> HHHHVKLSVVEQAPVVEGLTPAHSLQHSIELARLADRLGYERFWVAEHHAEIFNAVPAPEILIARIAAETSGIRVGSGGVLLSLYSPLKVAEVFRTLHALYPDRIDLGIGRANRVKLPVFAALRDDTAGKEPSSD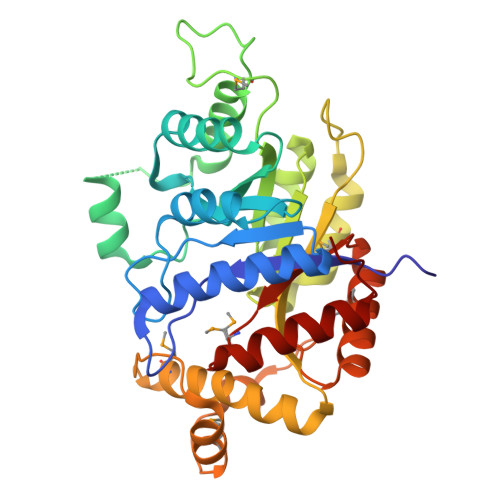DLWRRLEQLRAYLDPDSGLPFTVSPRMPGGPALWLLGASVSSADAAARLGLPYAYAHFITPDFTREAMDTYRAAFVPGPDTPSPRPILSVVVCCAETDAEAQRVYATHRLFHRRMSQGDVRLLPPADLAVAEMDKPGPDPLAEESFEWPRYVVGSPDRVRDQLTKMADATGAEELGVVSMIHDQRDRLRSYRLLAEAFELTPR>[3x]GSSMSAPTNLEQVLAAGGNTVEMLRNSQIGAYVYPVVAPEFSNWRTEQWAWRNSAVLFDQTHHMVDL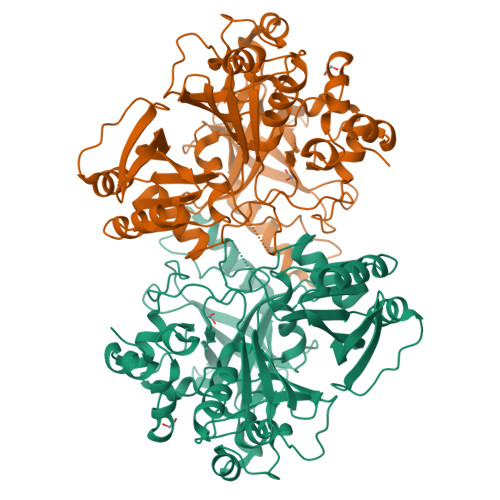YIRGKDALKLLSDTMINSPKGWEPNKAKQYVPVTPYGHVIGDGIIFYLAEEEFVYVGRAPAANWLMYHAQTGGYNVDIVHDDRSPSRPMGKPVQRISWRFQIQGPKAWDVIEKLHGGTLEKLKFFNMAEMNIAGMKIRTLRHGMAGAPGLEIWGPYETQEKARNAILEAGKEFGLIPVGSRAYPSNTLESGWIPSPLPAIYTGDKLKAYREWLPANSYEASGAIGGSFVSSNIEDYYVNPYEIGYGPFVKFDHDFIGRDALEAIDPATQRKKVTLAWNGDDMAKIYASLFDTEADAHYKFFDLPLANYANTNADAVLDAAGNVVGMSMFTGYSYNEKRALSLATIDHEIPVGTELTVLWGEENGGTRKTTVEPHKQMAVRAVVSPVPYSVTARETYEGGWRKAAVTA> FKQGQGMFSHQLKRLLQKKSIHRYNWDPLPMYDPRKLVHASRHMDVETWREVPD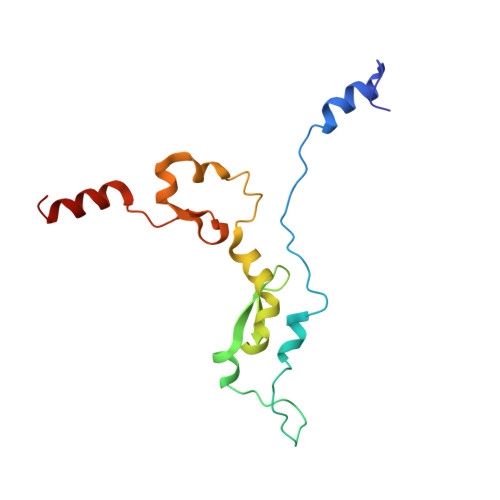PHWDERSYLVPDQMFYNIPVPPEYKDAYWWRELQARRVQCPVEWVSHRMYNKGDRQRYDFQDLAFRKKFEFSYEEVVKNAKDMRS>MSKIFDLVVIGAGSGGLEAAWNAATLYKKRVAVIDVQMVHGPPFFSALGGTCVNVGCVPKKLMVTGAQYMEHLRESAGFGWEFDRTTLRAEWKKLIAVKDEAVLNINKSYEEMFRDTEGLEFFLGWGSLESKNVVNVRESADPASAVKERLETENILLASGSWPHMPNIPGIEHCISSNEAFYLPEPPRRVLTVGGGFISVEFAGIFNAYKPKDGQVTLCYRGEMILRGFDHTLREELTKQLTANGIQILTKENPAKVELNADGSKSVTFESGKKMDFDLVMMAIGRSPRTKDLQLQNAGVMIKNGGVQVDEYSRTNVSNIYAIGDVTNRVMLTPVAINEAAALVDTVFGTNPRKTDHTRVASAVFSIPPIGTCGLIEEVASKRYEVVAVYLSSFTPLMHNISGSKYKTFVAKIITNHSDGTVLGVHLLGDNAPEIIQGVGICLKLNAKISDFYNTIGVHPTSAEELCSMRTPSYYYVKGEKMEKPSEASL[4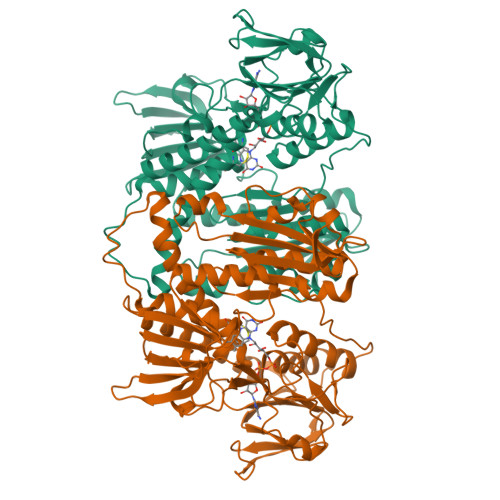x]5-{4-[(Z)-2-hydroxyethenyl]phenyl}-1-methyl-6-{[(1R)-1-phenylethyl]sulfanyl}-1,5-dihydro-4H-pyrazolo[3,4-d]pyrimidin-4-one | C22 H22 N4 O2 S | 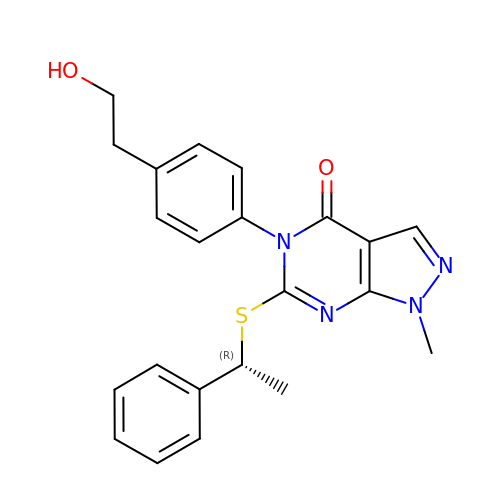ZYDLSTYFDFDODX-OAHLLOKOSA-N>[22x]MNQKHSSDFVVIKAVEDGVNV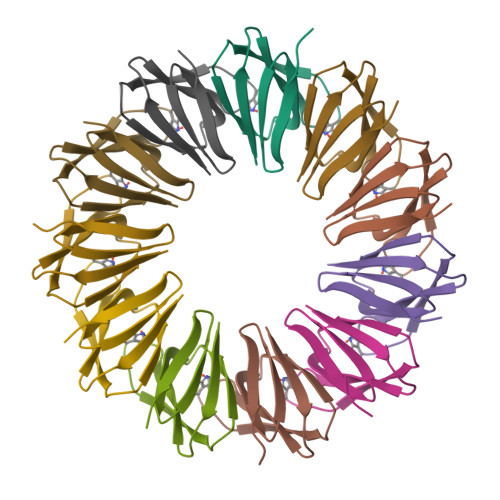IGLTRGTDTKFHHSEKLDKGEVIIAQFTEHTSAIKVRGEALIQTAYGEMKSEKK> MIVSAIAANALLESVTKFHCGVIYDYSTAEYVSYRPSDFGAYLDALEAEVARGGLIVFHNGHKYDVPALTKLAKLQLNREFHLPRENCIDTLVLSRLIHSNLKDTDMGLLRSGKLPGKRFGSHALE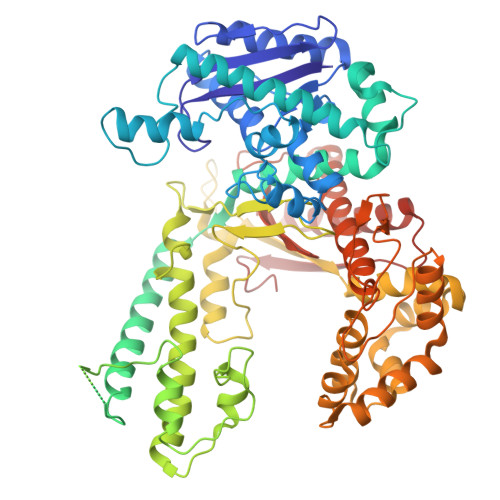AWGYRLGEMKGEYKDDFKRMLEEQGEEYVDGMEWWNFNEEMMDYNVQDVVVTKALLEKLLSDKHYFPPEIDFTDVGYTTFWSESLEAVDIEHRAAWLLAKQERNGFPFDTKAIEELYVELAARRSELLRKLTETFGSWYQPKGGTEMFCHPRTGKPLPKYPRIKTPKVGGIFKKPKNKAQREGREPCELDTREYVAGAPYTPVEHVVFNPSSRDHIQKKLQEAGWVPTKYTDKGAPVVDDEVLEGVRVDDPEKQAAIDLIKEYLMIQKRIGQSAEGDKAWLRYVAEDGKIHGSVNPNGAVTGRATHAFPNLAQIPGVRSPYGEQCRAAFGAEHHLDGITGKPWVQAGIDASGLELRCLAHFMARFDNGEYAHEILNGDIHTKNQIAAELPTRDNAKTFIYGFLYGAGDEKIGQIVGAGKERGKELKKKFLENTPAIAALRESIQQTLVESSQWVAGEQQVKWKRRWIKGLDGRKVHVRSPHAALNTLLQSAGALICKLWIIKTEEMLVEKGLKHGWDGDFAYMAWVHDEIQVGCRTEEIAQVVIETAQEAMRWVGDHWNFRCLLDTEGKMGPNWAICH>MAAEPLTELEESIETVVTTFFTFARQEGRKDSLSVNEFKELVTQQLPHLLKDVGSLDEKMKSLDV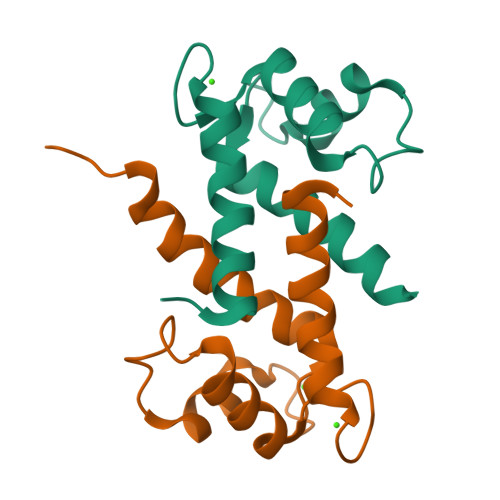NQDSELKFNEYWRLIGELAKEIRKKKDLKIRKK[2x]> MPVITLPDGSQRHYDHAVSPMDVALDIGPGLAKACIAGRVNGELVDACDL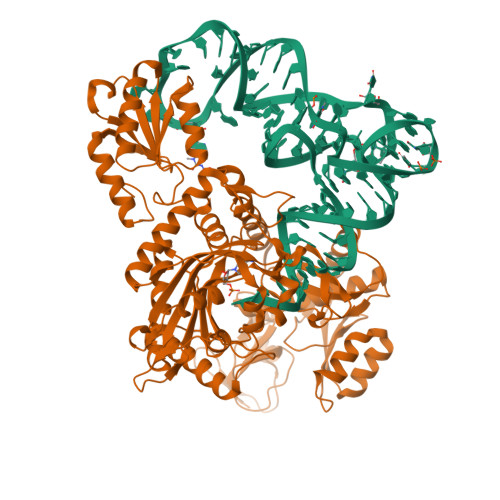IENDAQLSIITAKDEEGLEIIRHSCAHLLGHAIKQLWPHTKMAIGPVIDNGFYYDVDLDRTLTQEDVEALEKRMHELAEKNYDVIKKKVSWHEARETFANRGESYKVSILDENIAHDDKPGLYFHEEYVDMCRGPHVPNMRFCHHFKLMKTAGAYWRGDSNNKMLQRIYGTAWADKKALNAYLQRLEEAAKRDHRKIGKQLDLYHMQEEAPGMVFWHNDGWTIFRELEVFVRSKLKEYQYQEVKGPFMMDRVLWEKTGHWDNYKDAMFTTSSENREYCIKPMNCPGHVQIFNQGLKSYRDLPLRMAEFGSCHRNEPSGSLHGLMRVRGFTQDDAHIFCTEEQIRDEVNGCIRLVYDMYSTFGFEKIVVKLSTRPEKRIGSDEMWDRAEADLAVALEENNIPFEYQLGEGAFYGPKIEFTLYDCLDRAWQCGTVQLDFSLPSRLSASYVGEDNERKVPVMIHRAILGSMERFIGILTEEFAGFFPTWLAPVQVVIMNITDSQSEYVNELTQKLSNAGIRVKADLRNEKIGFKIREHTLRRVPYMLVCGDKEVESGKVAVRTRRGKDLGSMDVNEVIEKLQQEIRSRSLKQLEE>GSHMNNDFNGKITLAITGASGASYAMRLIECLIAANYQLYILCSSAGRIVLDTEVGVKIPSSPDAASKFLTEKYQAKDQQITVFGKEQWFSPVASGSSAPKQMVVCPCSTGTMAAICHGMSDNLIERAA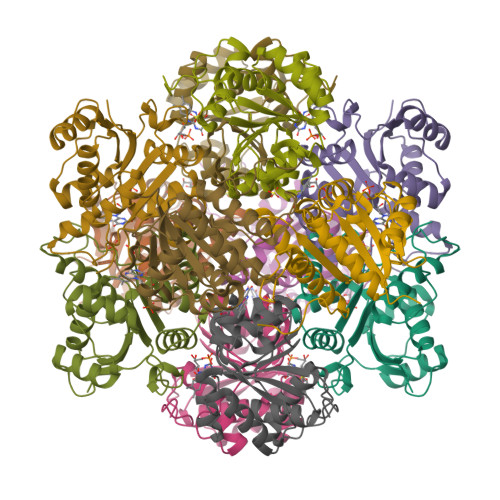DVVIKERGQLILMVRETPFSTLHLQNMLSLSQQGVTIMPASPGFYHKVETIEDLIDFMVGRVLDHLGIEQDIMPRWGYNI[6x]>MHLQIALFLVVVSLLVNVEAVPAKAQSDYVVSFRHIGRLLRDEREERGVSANAVETITDAVESKINTAQLKSWLESGESADDVFKLLKLDSAADKVLGHAKLDEWIEYMKLFNGQKGSKKTTLIKTLTAHFEDDGVARMIQKALQVDSTAKMAKRLQFEQIQRWLGQEKTPEEVLTLLKLDINRYDLFEKPELLTWVKYLDDWNKMYPDRQTTLFARISPLLEEGILANMLIKAKSVASTEKIALRIQAEQTASWLKAEKTPDDLFTLLRLNRAEDSPLLENPIFDAWVKYADDFREMYPKVSFDPIATISEHYTAAQVATMIVEAS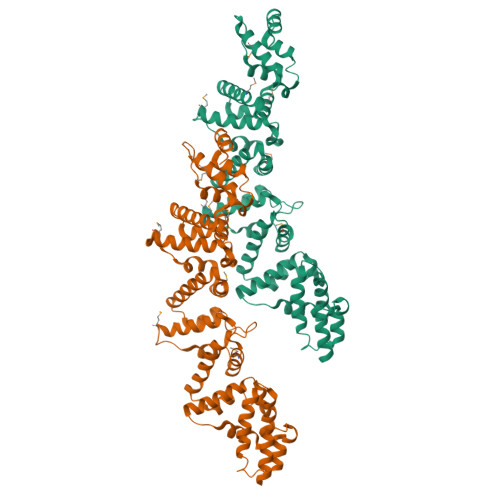KSPSTSSIAHRLNTEQFRDWLNTRQSPVRVFKLLKLDEAGDKLFQSPVITTWLNYATFYSTKREKVSITTLLRKRFGDEVLAGILTDAQQVPATKEEATKLLTSLVGRWPKSRVHPDNVYKWLRVEGREKTDGFRLFYERYAAAYKAARNG[2x]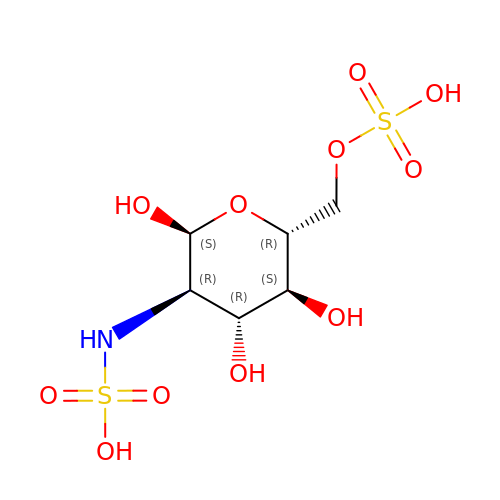2-deoxy-6-O-sulfo-2-(sulfoamino)-alpha-D-glucopyranose | C6 H13 N O11 S2 | DQTRACMFIGDHSN-UKFBFLRUSA-N>[6x]VEYKNTICPPRQDYRYWYFVAELTIGVNYDINSTIIGECHMSESYIDRNANIVLTGYGLKINMTIMDTDQRFVAAAEGVGKDNKLSVLLFTTQRLDKVHHNISVTITCMEMNCGTTKYNSDLPESIHKSSSCDITINGSCVTCVNLETDPTKINPHYLHPKNKYLYHNSEYSMRGSYGVTFIDELNQCLLDIKELSYDICYRE;>LKIQAYFNETADLPCQFANSQNQSLSELVVFWQDQENLVLNEVYLGKEKFDSVHSKYMGRTSFDSDSWTLRLHNLQIKDKGLYQCIIHHKKPTGMIRIHQMNSELSVLANFSQPEIVPISNITENVYINLTCSSIHGYPEPKKMSVLLRTKNSTIEYDGVMQKSQDNVTELYDVSISLSVSFPDVTSNMTIFCILETDKTRLLSSPFSIELED[6x]

Poxvirus encoded M2 protein is a member of the poxvirus immune evasion family and plays roles in host immunomodulation via the regulation of innate immune response mediated by the NF-κB pathway and adaptive immune response mediated by B7 ligands. Here we reveal that MPXV M2, co-existing as a hexamer and a heptamer, recognizes human B7.1 and B7.2 (hB7.1/2) with high avidities. The binding of oligomeric MPXV M2 interrupts the interactions of hB7.1/2 with CD28 and CTLA4 and subverts T cell activation mediated by B7.1/2 costimulatory signals. Cryo-EM structures of M2 in complex with hB7.1/2 show that M2 binds to the shallow concave face of hB7.1/2 and displays sterically competition with CD28 and CTLA4 for the binding to hB7.1/2.

We finally determined three complex structures, M2-hB7.1 hexamer, M2-hB7.2 hexamer, and M2-hB7.2 heptamer, at an overall resolution of 3.04, 2.7, and 3.12 Å, respectively. The resulting structures reveal that M2 forms an oligomeric ring structure with B7 proteins binding to the outer face of the M2 ring in a 1:1 stoichiometry. Structural analysis reveals that M2 interacts with hB7.1 and hB7.2 similarly. The interfaces of the two complex structures have very similar atomic contacts and bury a total accessible surface area of 1760 and 1617 Å2, respectively. M2 binds to hB7.1/2 side-by-side via β-strand complementation mediated by the C-terminal half of the M2 β11 and the N-terminal part of the hB7.1/2 G strand. The long C-terminal loop of M2 sits on top of the shallow concave surface, formed by the natural twist of strands G, F, C, and C’ of hB7.1/2. Extensive residues from the C-terminal loop, β8-β9 loop, and β10-β11 loop, and to a lesser extent, the β8, β9, β10, and β11 strands form a network of both van der Waals and hydrogen bonding interactions with residues from strands G, F, C, and C’ of hB7.1/2. Specifically, residues E122, K123, F126, K127, R128, and E133 from hB7.1, and residues M120, R122, Q125 as well as N127 from hB7.2 form hydrogen bonds with corresponding residues of M2 protein. For hB7.2, CTLA4 makes 14 contacts with hB7.2 and M2 makes 15 contacts with hB7.2, with 8 of these being shared residues. Surprisingly, the binding ability and half-life of M2 with hB7.1/2 significantly increased in this setting, leading to a KD of 0.15 nM and t1/2 of 397 min for hB7.1-M2 complex and a KD of 0.05 nM and t1/2 of 1180 min for hB7.2-M2 complex, respectively.>[4x]MRGSHHHHHHGSACELGTMPHIDNDVKLDFKDVLLRPKRSTLKSRSEVDLTRSFSFRNSKQTYSGVPIIAANMDTVGTFEMAKVLCKFSL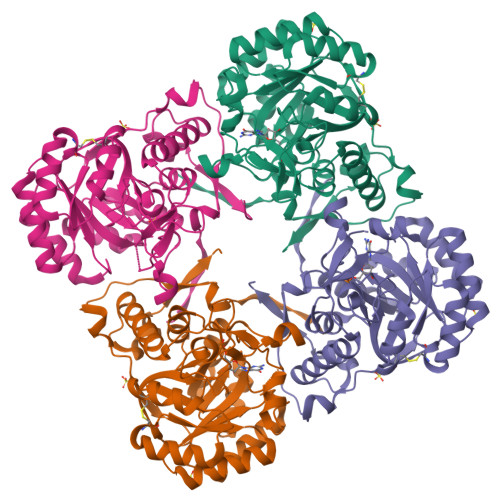FTAVHKHYSLVQWQEFAGQNPDCLEHLAASSGTGSSDFEQLEQILEAIPQVKYICLDVANGYSEHFVEFVKDVRKRFPQHTIMAGNVVTGEMVEELILSGADIIKVGIGPGSVCTTRKKTGVGYPQLSAVMECADAAHGLKGHIISDGGCSCPGDVAKAFGAGADFVMLGGMLAGHSESGGELIERDGKKYKLFYGMSSEMAMKKYAGGVAEYRASEGKTVEVPFKGDVEHTIRDILGGIRSTCTYVGAAKLKELSRRTTFIRVTQQVNPIFSEAC>[2x]HHHHHHYMEQEEDWDRDLLLDPAWEKQQRKTFTAWCNSHLRKAGTQIENIEEDFRNGLKLMLLLEVISGERLPRPDKGKMRFHKIANVNKALDFIASKGVKLVSIGAEEIVDGNLKMTLGMIWTIILRFAIQDISVEETSAKEGLLLWCQRKTAPYRNVNVQNFHTSWKDGLALCALIHRHRPDLIDYAKL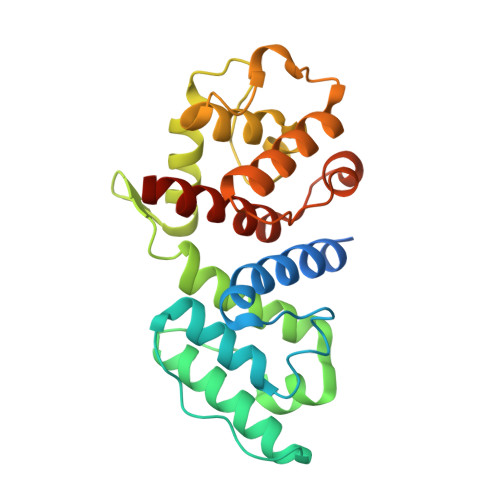RKDDPIGNLNTAFEVAEKYLDIPKMLDAEDIVNTPKPDEKAIMTYVSCFYHAFAGAEQAETAA> MGGDLTVKMLGGQEILVPLRDSMTVSELKQFIAQKINVPAFQQRLAHLDSREV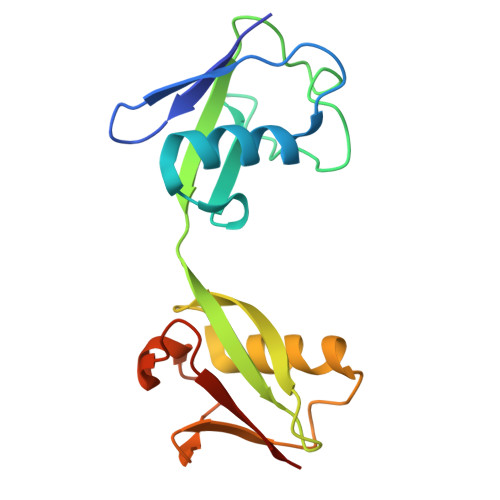LQEGVPLVLQGLRAGSTVLLVVQNSISILVRNDKGRSSPYEVQLKQTVAELKQQVCQKERVQADQFWLSFEGRPMDDEHPLEEYGLMKGCTVFMNLRLRGG The selective capture and retrieval of ER luminal proteins is controlled by the KDEL receptor (KDELR), which recognizes a specific ER-retrieval signal sequence (ERS) Lys-Asp-Glu-Leu (KDEL) at the C terminus of cargo proteins. Crystal structures of the chicken KDELR revealed a seven transmembrane (TM) spanning integral membrane protein with structural homology to the PQ-loop superfamily of membrane transporters. In the mildly acidic environment of the Golgi, KDEL-containing ER luminal proteins bind the receptor with high affinity, which elicits a signal for the integration of receptor-cargo complexes into COPI vesicles. In contrast, the neutral pH of the ER results in cargo release and the subsequent relocation of the empty receptor back to the Golgi, resetting the retrieval cycle.

We first sought to obtain structural insights into the transient ER form of the KDELR-cargo complex, which exists following delivery from the acidic environment of the Golgi. To capture a ligand-bound structure of the chicken KDELR at neutral pH, we took advantage of the higher affinity observed for the TAEHDEL peptide compared to the TAEKDEL variant, KD 0.24 μM vs. KD 1.94 μM, respectively. Crystals of the KDELR bound to the TAEHDEL peptide were grown at pH 7.0 using the lipidic cubic phase method and diffracted X-rays to 2.6Å. The receptor adopts the active state, with TM7 kinked out exposing the di-lysine COPI retrieval signal. Previous structural studies on the KDELR bound to either TAEKDEL or TAEHDEL peptides revealed two ordered water molecules (W1 and W2) at the base of the binding cavity. However, in the structure determined at pH 7.0, only one of the two water molecules (W2) is visible in the electron density maps. For structures at acidic pH, the water molecule at pH 7.0 coordinates interactions between His12, Tyr67 and Tyr162 on TM2 and TM6, respectively, and Asp9 on TM1 and does not interact with the carboxy-terminus of the TAEHDEL peptide. The loss of the W1 water molecule in the pH 7.0 structure thus collapses the hydrogen bond interaction network observed under acidic conditions, with the carboxy-terminus of the TAEHDEL peptide now only interacting with Arg47 and Arg159. At neutral pH, where only one water was resolved and the His12 has zero overall charge, there are two possible locations for the proton – either on the Nδ (HID) or on the Nϵ nitrogen (HIE). Therefore, HIE is the most likely state at pH 7.

> MNIFRLTGDLSHLAAIIILLLKIWKSRSCAGISGKSQLLFALVFTTRYLDLFTSFISLYNTSMKLIYIACSYATVYLIYMKFKATYDGNHDTFRVEFLIVPVGGLSFLVNHDFSPLEILWTFSIYLESVAILPQLFMISKTGEAETITTHYLFFLGLYRALYLVNWIWRYYFEGFFDLIAVVAGVVQTVLYCDFFYLYVTKVLKGKKLSLPA;> TAEHDEL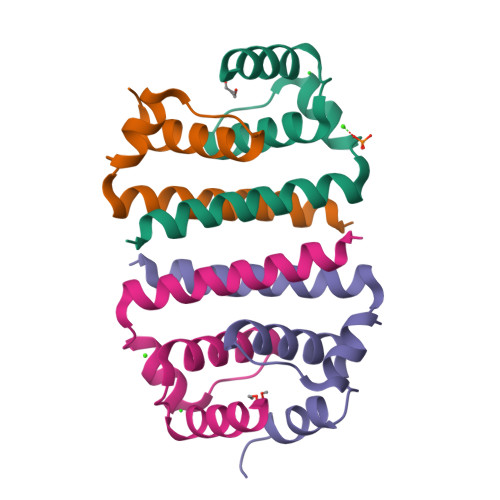>[8x]RVLSLTGLKRAMLSLIDGRGPTRFVLALLAFFRFTAIAPTRAVLDRWRSVNKQTAMKHLLSFKKELGTLTSAINRR> SGIPMKQMDLELPRFSYYPVVKPEPLSKQDTDILSNYINPLYLTPDGIEKLSKRFFQDSVIVLVEFLNQEFANTLLKRIIDAERQPTPMHSSEVSFPWKTAIPPHKHRYLYLDHEEFGPDIILPMDLQRLPAFQRWIQLVSGLPLRSFHQVGRRFRPGSDFTLATTNDTALL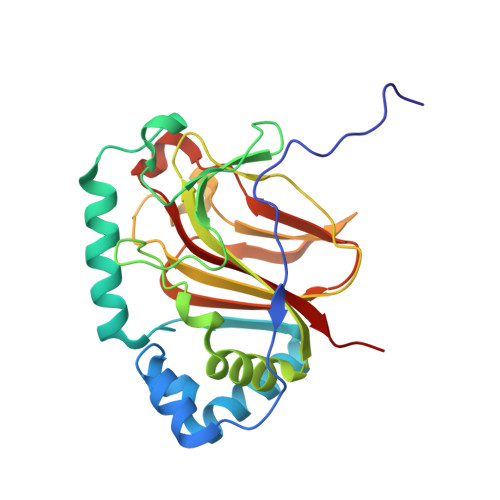EATLCLSPGTGIANTDNGAYDIYMIGDEDPDVDAAVYRGDQQDDSILLSLPAAWNVFSLVYRDEGVLQFVKYVSRQAESSRWDIYSQWNPVAE>[4x]HHHHHHMSAIK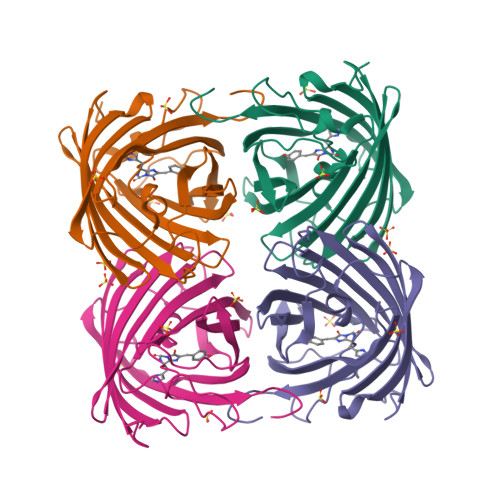PDMKINLRMEGNVNGHHFVIDGDGTGKPFEGKQSMDLEVKEGGPLPFAFDILTTAFHYGNRVFAEYPDHIQDYFKQSFPKGYSWERSLTFEDGGICIARNDITMEGDTFYNKVRFHGVNFPANGPVMQKKTLKWEPSTEKMYVRDGVLTGDITAALLLEGNAHYRCDSRTTYKAKEKGVKLPGYHLVDHCIEILSHDKDYNKVKLYEHAVAHSGLPDNARR>MGSIGEPNRLLCWSIYVTKK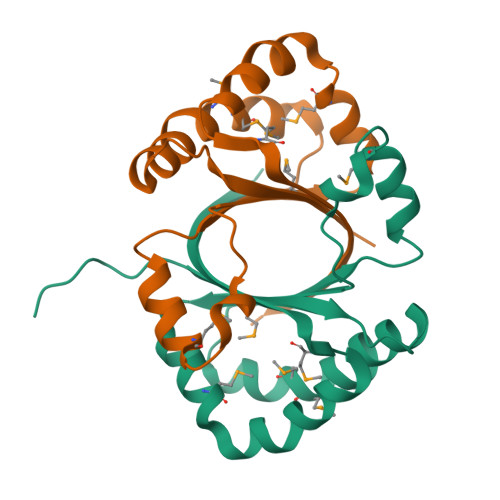PDQSEEDHHNHVSKVNAPMMIPFLKKYGIVRYTVKHNDAYSKPKQAALMAGQPEENVLAYDTVFEMIVKDIESIQTMQKDEEFLRTTIPDHFNFADMTRSKGSLTWIEEFTFALEHHHHHH[8x]> QQAGTATAENHPPLTWQECTAPGSCTTQNGAVVLDANWRWVHDVNGYTNCYTGNTWDPTYCPDDETCAQNCALDG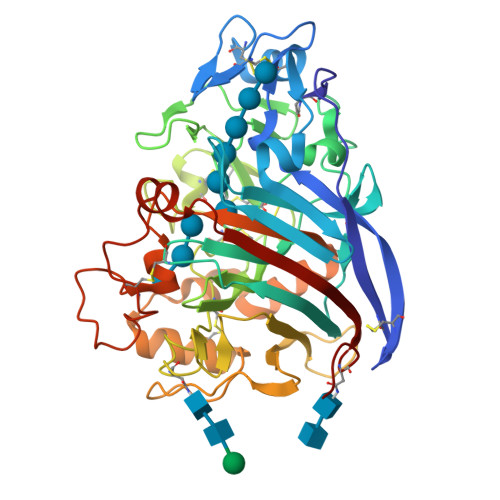ADYEGTYGVTSSGSSLKLNFVTGSNVGSRLYLLQDDSTYQIFKLLNREFSFDVDVSNLPCGLNGALYFVAMDADGGVSKYPNNKAGAKYGTGYCDSQCPRDLKFIDGEANVEGWQPSSNNANTGIGDHGSCCAEMDVWEANSISNAVTPHPCDTPGQTMCSGDDCGGTYSNDRYAGTCDPDGCDFNPYRMGNTSFYGPGKIIDTTKPFTVVTQFLTDDGTDTGTLSEIKRFYIQNSNVIPQPNSDISGVTGNSITTEFCTAQKQAFGDTDDFSQHGGLAKMGAAMQQGMVLVMSLWDDYAAQMLWLDSDYPTDADPTTPGIARGTCPTDSGVPSDVESQSPNSYVTYSNIKFGPINSTFTAS> TGSAKLECPQDWLSHRDKCFHV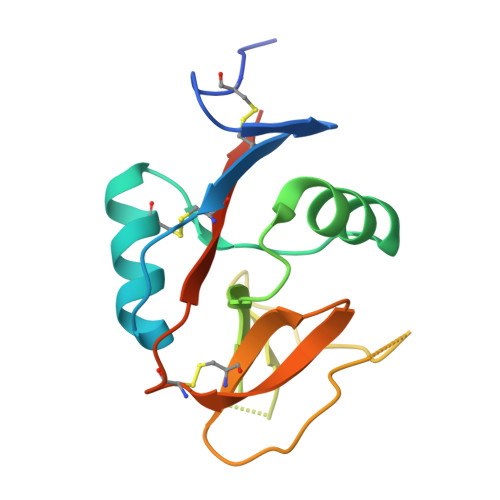SQVSNTWKEGRIDCDKKGATLLLIQDQEELRFLLDSIKEKYNSFWIGLSYTLTDMNWKWINGTAFNSDVLKITGVTENGSCAAISGEKVTSEGCSSDNRWICQKELNGTHHHHHH> SIVTKSIVNADAEARYLSPGELDRIKSFVTSGERRVRIAETMTGARERIIKQAGDQLFGKRPDVVSPGGNAYGAD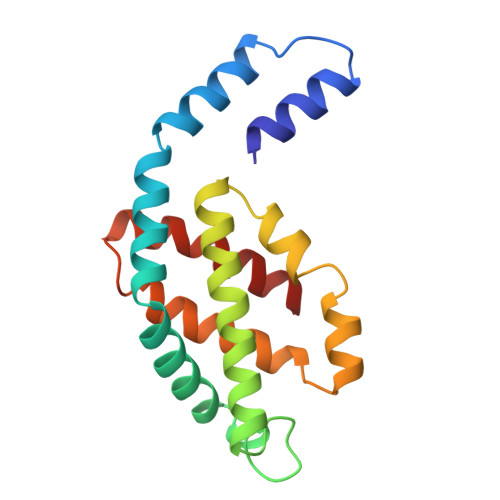MTATCLRDLDYYLRLITYGIVAGDVTPIEEIGVVGVREMYKSLGTPIEAIAEGVRAMKSVATSLLSGADAAEAGSYFDYLIGAMS Central to this ability are non‐canonical covalent intramolecular crosslinks between protein side chains forming isopeptide, thioester, and ester bonds that impart remarkable stability enhancement to single adhesin protein domains or are involved directly in covalent adhesion to host cells (Alegre‐Cebollada et al. 2010; Kang et al. 2007; Kang and Baker 2009; Kwon et al. 2014; Lei et al. 2021; Miller et al. 2018; Pointon et al. 2010; Walden et al. 2015). The autocalytic machinery of ester bond crosslinking, as first exemplified in the Clostridium perfringens adhesin Cpe0147, shows three residues (D577/H572/T450) arranged in space to mimic the acid/base/nucleophile catalytic triad of a serine protease, with Q580 the equivalent of a substrate electrophile (Kwon et al. 2014; Schwarz‐Linek and Banfield 2014). Two buried and protonated acids, D480 and E547, act like the oxyanion site of a serine protease, polarizing the carbonyl bond of Q580 side chain to increase its electrophilic potential and reactivity, and potentially stabilizing a high‐energy tetrahedral intermediate. In the proposed mechanism, H572 abstracts a proton from T450 Oγ1, which then effects nucleophilic attack on the Q580 Cδ with the loss of the side chain amino group as ammonia—the final state is the equivalent of the acyl‐intermediate of a serine protease mechanism, but without the potential to hydrolyze it is essentially trapped.

The replacement of the nucleophile threonine with a serine produces a crosslink species that is then hydrolysable at basic pH, and we have further proposed that this reaction follows the second half of a serine protease mechanism, whereby a water molecule attacks and breaks the ester bond of the acyl‐intermediate (Young et al. 2017). The T450S protein, similarly to T450C, closely resembles the wild type with an RMSD comparison of 0.66 Å across all Cα atoms. An intramolecular ester bond linking S450 and Q580 is unambiguously present. The pocket occupied by the T450 methyl group in the wild type or thiol in the T450C mutant is partly occupied by the buried acid E547, which, having rotated outwards from the wild‐type localization, no longer forms a proton shuttle with D480 and the ester bond carbonyl. Instead, E547 hydrogen bonds to an adjacent backbone carbonyl of V110 and stacks directly above the ester bond ether oxygen, making a close contact (E547 Oε1–S450 Oγ, 3.2 Å). The T450S structure instead shows the E547 side chain rotated out of the protein interior and stacking directly above the ester bond ether's oxygen (Ser‐450 Oγ). With respect to the mechanism of hydrolysis, as shown in the T450S crystal structure and reiterated by metadynamics simulations, the presence of the smaller serine relative to threonine considerably increases the likelihood of E547 directing its carboxyl group outward and close to the ether oxygen of the ester bond. T → S substitution enhances the ability of E547 to swing towards the ester bond to facilitate hydrolysis.

> GAMDPEFNLPEVKDGTLRSTVIADGVNGSSEKEALVSFENSKDGVDVKDTINYEGLVANQNYTLTGTLMHVKADGSLEEIATKTTNVTAGENGNGTWGLDFGNQKLQVGEKYVVFENAESVENLIDTDKDYNLDTKQVVKHEDKNDKAQTLVVEKP>SNAMPVVKINAIEVPAGAGPELEKRFAHRAHAVENSPGFLGFQLLRPVKGEERYFVVTHWESDEAFQAWANGPAIAAHAGHRANPVATG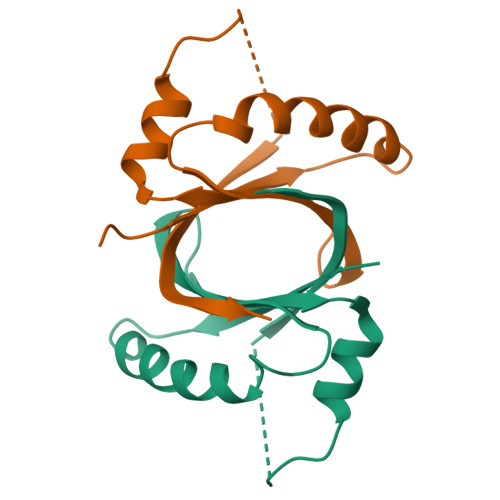ASLLEFEVVLDVGGTGKTA[2x]Purine nucleoside phosphorylases (PNPs, EC 2.4.2.1) are cytosolic enzymes involved in the purine salvage pathway metabolism in most organisms. The enzyme degrades (2′-deoxy)nucleosides based on 6-oxopurines to the corresponding purine bases and (2-deoxy)ribose-1-phosphate. Purine nucleoside phosphorylase (PNP) is a well-known molecular target with potential therapeutic applications in the treatment of T-cell malignancies and/or bacterial/parasitic infections. The results are supported by a crystallographic study of eight enzyme-inhibitor complexes and by ADMET profiling in vitro and in vivo.

To obtain information on the binding pose and interacting residues, crystal structures of recombinant hPNP in complex with inhibitors 18c, 45b, 45q, 45i, and 45n were determined and refined to high resolution. Bulky, fluorinated-phenyl substituent at position C4 of 45i interacts with helix by forming a halogen bond with the carbonyl group of the Val260 main chain as well as van der Waals and other interactions with other residues in the helix such as Leu261 and Gly264. The addition of bulky substituents at phenyl positions C4 and C5 in 45i and 45n both lead to a 2-fold decrease in affinity toward hPNP, compared to 18c. Compounds 45i and 45n, however, have quite distinct poses within the active site: major differences between the position of the central phenyl moiety as well as substituents are observed. While both bulky substituents extend toward the helix, their poses are quite different, and each makes different interactions with helix residues. The structural explanation for comparable affinities of 45i and 45n is the flexibility of the phenyl-moiety binding pocket that enables to accommodate moiety shifts and by the substantial shift of helix to adjust to the position of the bulky substituents at position C4. Crystals of hPNP/45i were prepared in a hanging drop using EasyXtal 15-Well Tool plates, with a 500 μL reservoir, which contained 1 M lithium sulfate, 100 mM tri-sodium citrate, and pH 5.4. Cubic crystals, dimensions 150 × 150 × 150 μm, appeared after 3 weeks and were harvested after 4 weeks.

>[3x]MENGYTYEDYKNTAEWLLSHTKHRPQVAIICGSGLGGLTDKLTQAQIFDYGEIPNFPRSTVPGHAGRLVFGFLNGRACVMMQGRFHMYEGYPLWKVTFPVRVFHLLGVDTLVVTNAAGGLNPKFEVGDIMLIRDHINLPGFSGQNPLRGPNDERFGDRFPAMSDAYDRTMRQRALSTWKQMGEQRELQEGTYVMVAGPSFETVAECRVLQKLGADAVGMSTVPEVIVARHCGLRVFGFSLITNKVIMDYESLEKANHEEVLAAGKQAAQKLEQFVSILMASIPLPDKAS>ANPCCSNPCQNRGECMSTGFDQYKCDCTRTGFYGENCTTPEFLTRIKLLLKPTPNTWHYILTHFKGVWNIVNNIPFLRSLIMKYVLTSRSYLIDSPPTYNVHYGYKSWEAF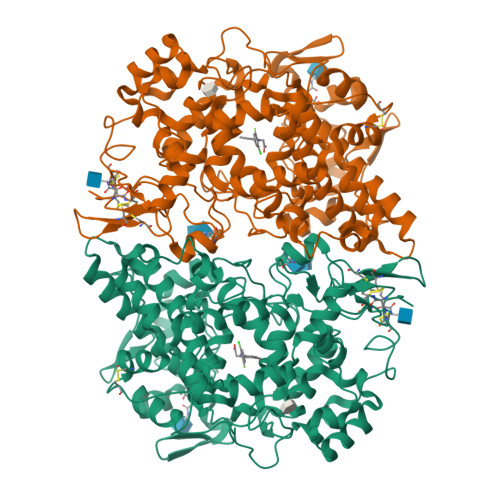SNLSYYTRALPPVADDCPTPMGVKGNKELPDSKEVLEKVLLRREFIPDPQGSNMMFAFFAQHFTHQFFKTDHKRGPGFTRGLGHGVDLNHIYGETLDRQHKLRLFKDGKLKYQVIGGEVYPPTVKDTQVEMIYPPHIPENLQFAVGQEVFGLVPGLMMYATIWLREHNRVCDILKQEHPEWGDEQLFQTSRLILIGETIKIVIEDYVQHLSGYHFKLKFDPELLFNQQFQYQNRIASEFNTLYHWHPLLPDTFNIEDQEYSFKQFLYNNSILLEHGLTQFVESFTRQIAGRVAGGRNVPIAVQAVAKASIDQSREMKYQSLNEYRKRFSLKPYTSFEELTGEKEMAAELKALYSDIDVMELYPALLVEKPRPDAIFGETMVELGAPFSLKGLMGNPICSPQYWKPSTFGGEVGFKIINTASIQSLICNNVKGCPFTSFNVQDPQPTKTATINASASHSRLDDINPTVLIKRRSTEL[2x]> XXXXXXXXXXXXXXXXXXXXXXXXXXXXXXXXXXXXXXGTVTVRLAASTHAEGTMIADALRRAHLVDGIPWSQMAVIVRSVPRVGTALARALTAAGVPVQDNGTDVPVGRQPAAAALLTVLDVTATGHLDADSAVALLTGPIGRVDPVTLRQLRRALRRADGSQPPRDFGDLLVDAIEREPKGLSAEHARTLRRLRAVLTAARRSDASGADPRYTLWQAWHASGLQRRWLAASERGGSVGAQADRDLDAVTTLFDVADQYVNRTAGASLRGLVDHVTRLGAAVARTEPETAAEAVAVLSVHGALAGEWDFVVIAGVQEGLWPNMIPRGGVLGTQHLVDVLDGVADMTDRTVSTRAPLVAEERRLLMAAMGRARTRVMITAVDSXXXXXXXXXXXXXPPLVAPRVLAPSALVGRLRAVVCAPDGAVDDDARACAAAQLARLAAAGVPGADPSQWHAMTSLTTEEPLWSEPGHVVTLSPSTLQMLTDCPLRWLLERHGGDDGRDVRSTVGSLVHALVSEPGKTESQLVNELEKVWDDLPYDAKWYSDNELARHRAMLETFTRWREDTRRQLTEVATEIPVEGIVVEPGENTPGVRVRGRLDRLERDEAGRLVVVDLKTGKSPVTKDDAQNHAQLAMYQLAVAAGLLDDGDEPGGGKLVYLGKAGAAGATEREQDPLTPDKRAEWLETVGEAAAATAGPRFVARVNNGCANCPVRSSCPAQANGDRP;> MTQVASPVVQARYSPVELSAALGLFPPTDEQAAVIAAPPGPLVVIAGAGAGKTETMAARVVWLVANGFATPSQVLGLTFTRKAAGQLLRRVRTRLARLAGAGLAPGSGASDESATVSTYHAFAGTLLREHGLLLPVEPDTRLLSETELWQLAYDVVCAHPGHLDTEKTPAAVTAMVLRLSGALAEHLVDTD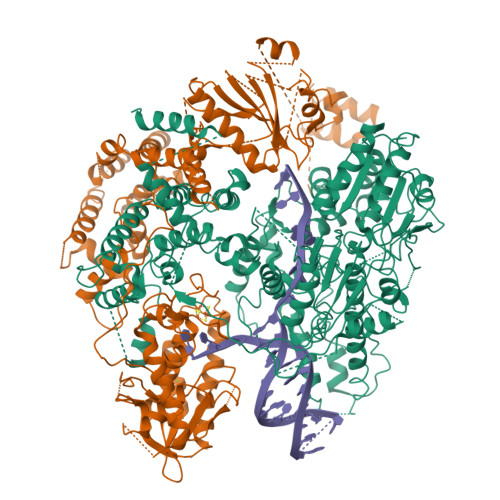QLRDTHVELERLVHTLPAGPYQRDRGPSQWLLRMLATQTERTELVPLIDALHQRMRAEKVMDFGMQMAAAARLAARFPQVGEQLRQRFRVVLLDEYQDTGHAQRIALSSLFGGGADDGLALTAVGDPIQSIYGWRGASATNLPRFTTDFPYSDGTPAPTLELRTSWRNPPSTLHVANAVSEEARRRSVAVRALRPRPDAEPGTIRCALLNNVAAERDWVADHLARAYHGAIGRGEAAPTAAVLVRRNADAAPMAEALTARGVPVEVVGVAGLLAVPEVADLVAMLRLIADPTAGSAVMRILTGPRWRFGARDIAALWRRAVELDDRPKGELGTADIVAQAAPDADTACVADAICDPGDAERYSPAGYERIVALGRELTMLRAHLGHPLPELVAEVRRVLGLDAEARAARPVAAGWAGTENLDRFSDLVSDFAGHAGASVSALLAYLDAAVEVENGLAPAELTVSHDRVQILTVHAAKGLEWQVVAVPHLSARVFPSTTQARTWLTDASDLPPLLRGDRATESEIGVPVLDTSDIYDRKILSDKISDHKKSLDQRRVDEERRLLYVAITRAEDTLLLSGHHWGATESKPRGPSEFLCELKTILEEATAAGTPCGEIEHWAPDPAPGETNPLRDQVVEALWPPVASADDHVHRGAQLVAAAMAGEVSAEADQEGWAADVDALLAERERPPQQEDTELPGQLSVSTLVELSRDPKAALTRLRRRLPQRPDPHALLGTTFHEWVQRYFHAERLFDLDDLPGAVDSDSGRAVEESLAELQDAFVKSPWAARTPVEVEVPFDMVLGETVVRGRIDAVFAEPDGTTMVLDWKTGDPPETPEAKEHAAVQLAVYRLAWAAMRGCPPESVRAAFHYVRSGQTVIPETLPGAEELVKLLAAAPTETAEEADRIT> 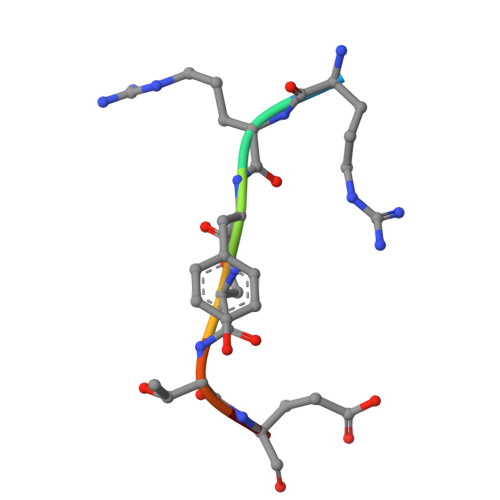RRYSTEL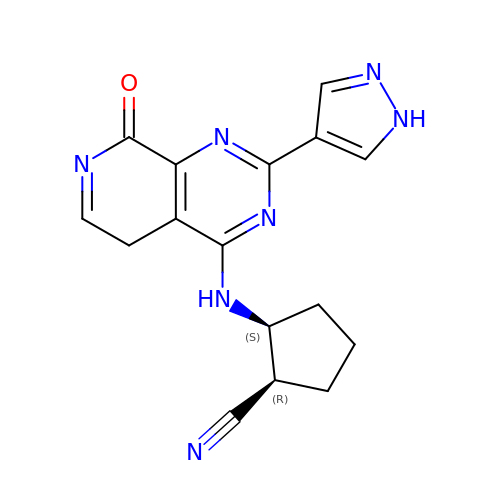(1R,2S)-2-{[8-oxo-2-(1H-pyrazol-4-yl)-5,8-dihydropyrido[3,4-d]pyrimidin-4-yl]amino}cyclopentanecarbonitrile | C16 H15 N7 O | GGNYHYINELGWQU-CABZTGNLSA-N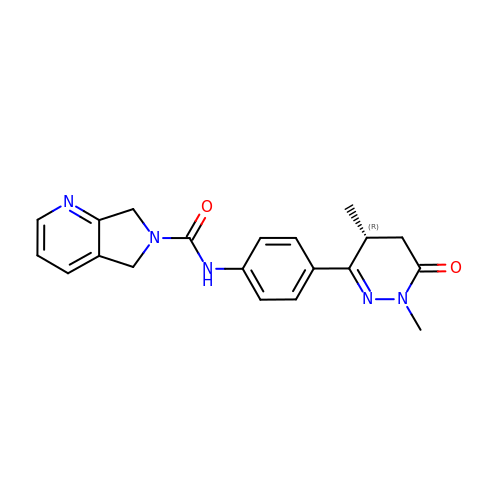N-[4-[(4R)-1,4-dimethyl-6-oxidanylidene-4,5-dihydropyridazin-3-yl]phenyl]-5,7-dihydropyrrolo[3,4-b]pyridine-6-carboxamide | C20 H21 N5 O2 | IJKUAZSSMFHECB-CYBMUJFWSA-N> TPVVINNSNVIVCEICKMAVKLIVPEADKDLDQLEKEFIQGCMTLIGWLPYAEKECKA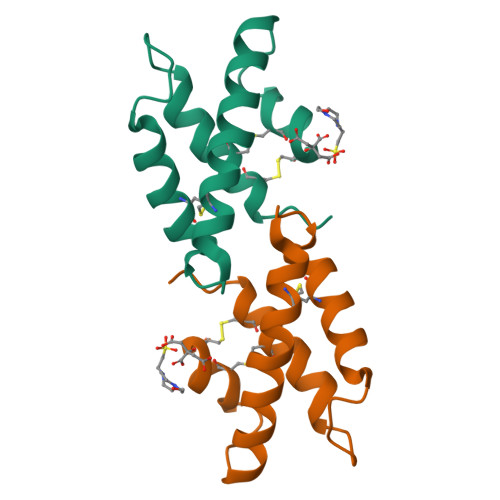LAKIEMGAIKTLLENGSAPEEICTTLHAC> GGSDPAISKDV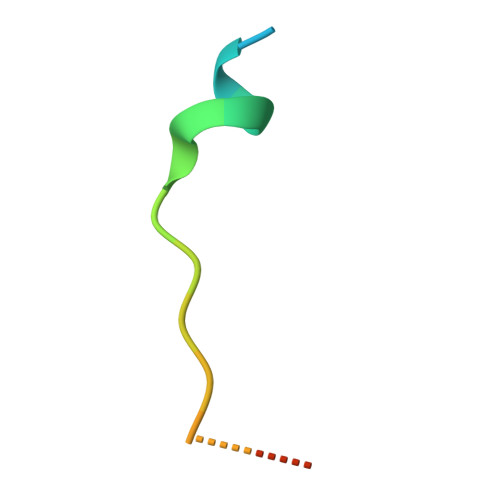VLSSSSFLRA> MGKRVLIVDDATNGREAVEKYKELKPDIVTMDITMPEMNGIDAIKEIMKIDPNAKIIVCSAMGQQAMVIEAIKAGAKDFIVNTAAVENPSLITQIAQTFGSQAVVVAIDAKRVDGEFMVFTYSGKKNTGILLRDWVVEVEKRGAGEILLTSIDRDGTKSGYDTE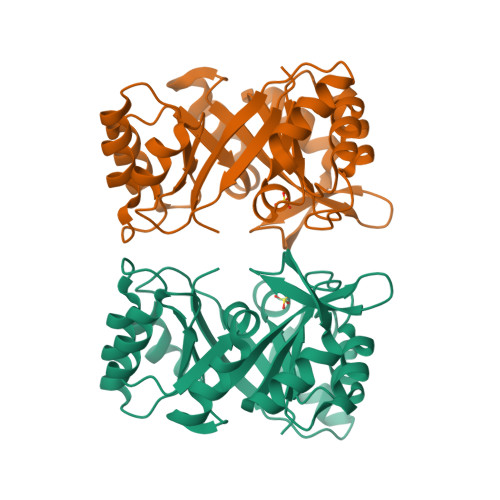MIRFVRPLTTLPIIASGGAGKMEHFLEAFLAGADAALAASVFHFREIDVRELKEYLKKHGVNVRLEGLLEHHH>MSILFSSILFSIATFFSRILGLFRDVLFAKYFGVSYELDAYFIAIMFPFFLRKVFGEGAMSSAFVPLYSEKSGEEKDKFLSSVINGFSLIILALVILSYFFPELIINLFGAGSSHETKILAKKLLLITSPSIYFIFLWAISYSILNTNNKFFWPALTPSISNITIIIGTFLSTKYGIISPTIGFLIGSILMFFSIIKSIIKHKYYFTIKHFPHFLKLFFPTFMTMVVSQINTVVDMNVVSFYDKGSISYLQYASRFYLLPYGLFAVSVSTVVLSKISNDRKNFNYHLNDALK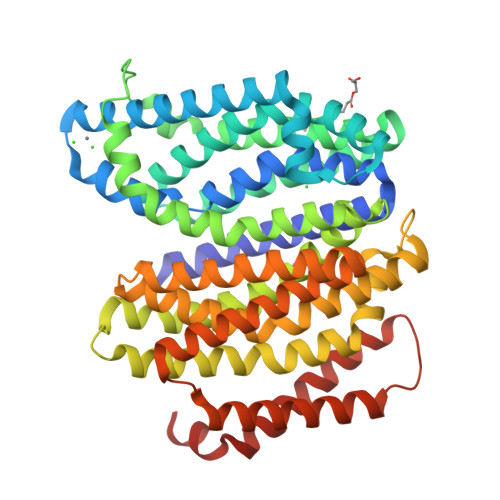TTLFFTIPSMVGLIFLSTPIIRFFYEHGAFTSKDTLITSKILIAYTLGLPFYGIYSTISRSYHAIKNTKTPFIAATIVSLSNIILDIIFGLKYGPIGVALATSIAGIIGVLYLLFSVKTFPIKDFLKISLNSLIMLFVIYLTDFTDNEFWFLIQILIGILVYLIFSSIFYRDLIRRFLYARKK[2x]>MGILQANRVLLSRLLPGVEPEGLTVRHGQFHQVVIASDRVVCLPRTAAAAARLPRRAAVMRVLAGLDLGCRTPRPLCEGSAEGAVELPFLVLSRVPGAPLEADALEDSKVAEVVAAQYVTLLSGLASAGADEKVRAALPAPQGRWRQFAADVRAELFPLMSDGGCRQAERELAALDSLPDITEAVVHGNLGAENVLWVRDDGLPRLSGVIDWDEVSIGDPAEDLAAIGAGYGKDFLDQVLTLGGWSDRRMATRIATIRATFALQQALSACRDGDEEELADGLTGYR[2x]

In this study, we focus on a resistance gene cph, which encodes a phosphotransferase (Cph) that confers resistance to the antituberculosis drug capreomycin (CMN). To confirm whether proteins in cluster I also confer resistance to CMN, three proteins, Cph001 from Streptosporangium roseum (accession number: WP_012891209), Cph002 from Streptomyces sp. SID8364 (MYT78782), and Cph003 from Streptomyces filamentosus NRRL15998 (EWS93654), were selected for disk diffusion assays. The polypeptide chain of Cph001 is folded into two domains, an N-terminal lobe domain (Met1–Gly97) and a C-terminal domain (Ala98–Arg286). The C-terminal domain further divided into a core subdomain (Ala98–Ala140 and Thr182–Ser246) and an α-helical subdomain (Pro141–Ile181 and Asp247–Arg286).

Based on the disk diffusion assay, E. coli harboring cph001 are resistant to VIO but not to Kan and Ery. Consistently, Cph001 is only capable of phosphorylating VIO, and thus Cph001 confers cross-resistance to the CMN analogous antibiotic VIO. Based on the disk diffusion assay and the couple enzyme assay mentioned previously, Cph001 confers cross-resistance to CMN and VIO. We then solved the crystal structure of Cph001D189N-VIO. The complex structures Cph001D189N-CMN IIA, Cph001D189N-CMN IIB, and Cph001D189N-VIO revealed that CMN and VIO occupy the same position with a similar conformation; the pentapeptide backbones are superimposed well while the β-lysine moiety is located on the opposite position between VIO and CMN. The β-lysine moiety of VIO extends into the α-helical subdomain while that of CMN extends towards the N-terminal lobe domain. Moreover, the additional hydroxyl group at the capreomycidine moiety of VIO points towards the protein surface without any specific interaction. The complex structure Cph001D189N-VIO supports cross-resistance of Cph001 and provides molecular details of VIO-binding environment. ITC analysis revealed that VIO binds to Cph001 with a KD value 4.18 ± 0.68 μM, which is similar to the KD value for binding of CMN IIA.>APQQGTNVNDKVHFSNIDIAIDKGHVNQTTGKTEFWATSSDVLKLKANYTIDDSVKEGDTFTFKYGQYFRPGSVRLPSQTQNLYNAQGNIIAKGIYDSTTNTTTYTFTNYVDQYT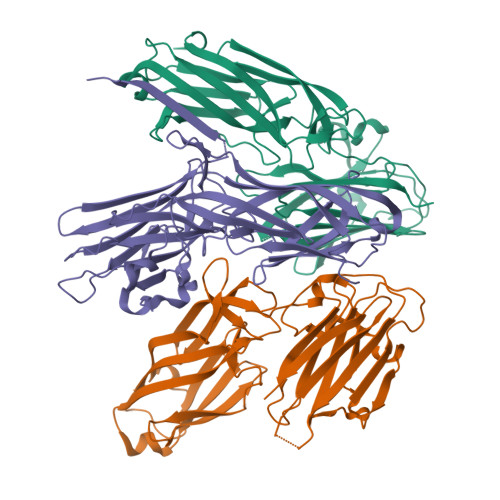NVRGSFEQVAFAKRKNATTDKTAYKMEVTLGNDTYSEEIIVDYGNKKAQPLISSTNYINNEDLSRNMTAYVNQPKNTYTKQTFVTNLTGYKFNPNAKNFKIYEVTDQNQFVDSFTPDTSKLKDVTDQFDVIYSNDNKTATVDLMKGQTSSNKQYIIQQVAYPDNSSTDNGKIDYTLDTDKTKYSWSNSYSNVNGSSTANGDQKK[3x]>[2x]LEEKKVCQGTSNKLTQLGTFEDHFLSLQRMFNNCEVVLGNLEITYVQRNYDL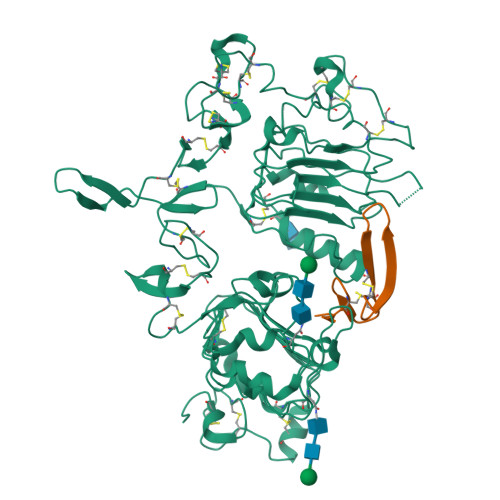SFLKTIQEVAGYVLIALNTVERIPLENLQIIRGNMYYENSYALAVLSNYDANKTGLKELPMRNLQEILHGAVRFSNNPALCNVESIQWRDIVSSDFLSNMSMDFQNHLGSCQKCDPSCPNGSCWGAGEENCQKLTKIICAQQCSGRCRGKSPSDCCHNQCAAGCTGPRESDCLVCRKFRDEATCKDTCPPLMLYNPTTYQMDVNPEGKYSFGATCVKKCPRNYVVTDHGSCVRACGADSYEMEEDGVRKCKKCEGPCRKVCNGIGIGEFKDSLSINATNIKHFKNCTSISGDLHILPVAFRGDSFTHTPPLDPQELDILKTVKEITGFLLIQAWPENRTDLHAFENLEIIRGRTKQHGQFSLAVVSLNITSLGLRSLKEISDGDVIISGNKNLCYANTINWKKLFGTSGQKTKIISNRGENSCKATGQVCHALCSPEGCWGPEPRDCVSHHHHHH;>[2x]SEGPIALKFSHLCLEDHNSYCINGACAFHHELEKAICRCFTGYTGERCEHLTLTSYAVDSY> MGSSHHHHHHSSGLVPRGSHAMADYTEQDAMRVQAVKTYIDNVLQEGRSQIKTTPLLADGINTTTRKPVEWIYPDGRTATISNFANQQNFLRALTAMSVVTEDQRYQLEAVRITRYFMDNFIADNGLFYWGGHRFVNLDTLELEGPQNKNSVHELKNHYPYYPFLYHVDPHATERYIKAFWQAHVEDWQSLDMGRHGSYSKNYDDKVFHRPIPASLVDQSKLPIMPETKGLTFINAGSDLIYAAYQLDWLAPSANAQGSAAWGQYLMTQYKLAKHPKTGAPVYQFTSPKKREWPPQSDKDTNSKYGDRAARQFGPELGNIAREGNVLFKSNDKSIVFNNALIELHLAEQRNDAAIREQVVDALLNFYRLAYNPENGTIKPIFSDGTSIEGIPLARDGYYGPKGRVFNAHKPKTEEYLLPILRAYRLQADPELWQLAANMTHHYGWGSLGNDAKAKPTLNMQLSSVSPMTLFSAIELYQITQQPEYLEFARAAADKLVEKRFVRGYFLAN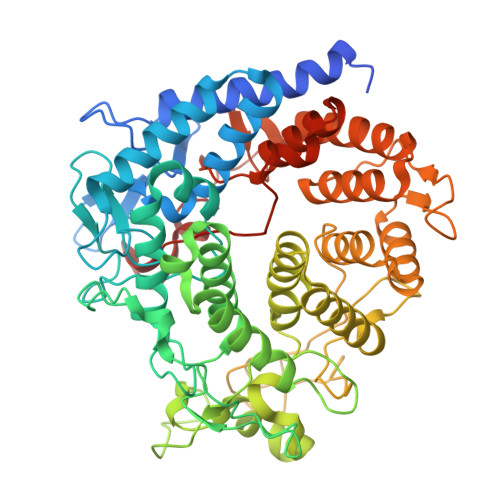PRYLNASIDAIEPLALLTLDATLKGKTAQVAPYLSGSGYIHGEFAGKENAYDTNEIYKQTR> GSPNNLETYEWYNKSISRDKAEKLLLDTGKEGAFMVRDSRTPGTYTVSVFTKAIISENPC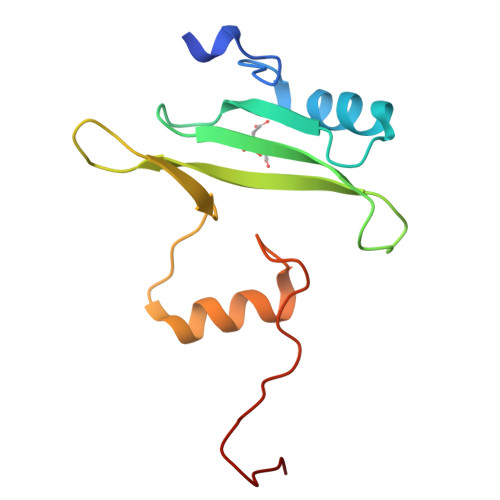IKHYHIKETNDSPKRYYVAEKYVFDSIPLLIQYHQYNGGGLVTRLRYPVCGSPGIHRD> GMGSIKEIAITHHVKEGHEKADPSQFELLKVLGQGSFGKVFLVKKISGSDARQLYAMKVLKKATLKVRDRVRTKMERDILVEVNHPFIVKLHYAFQTEGKLYLILDFLRGGDLFTRLSKEVMFTEEDVKFYLAELALALDHLHSLGIIYRDLKPENILLDEEGHIKLTDFGLSKESIDHE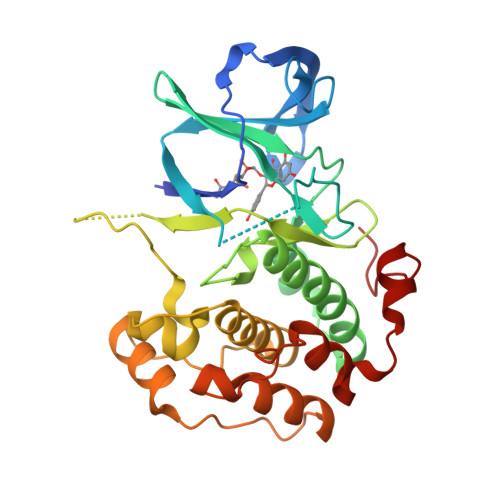KKAYSFCGTVEYMAPEVVNRRGHTQSADWWSFGVLMFEMLTGTLPFQGKDRKETMTMILKAKLGMPQFLSPEAQSLLRMLFKRNPANRLGAGPDGVEEIKRHSFFSTIDWNKLYRREIHPPFKP(2S)-1-hydroxy-3-(tetradecanoyloxy)propan-2-yl docosanoate | C39 H76 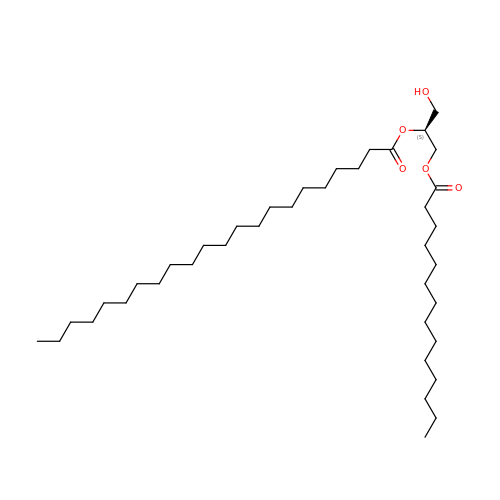O5 | DINFAYNBAABMIP-QNGWXLTQSA-N> MRFVMPGDRIGSAEEYVKGEGVYEEGGELFAAVA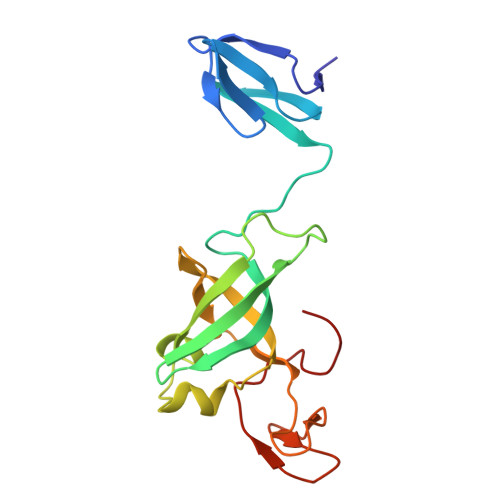GKLIIKDRVAKVESISPIPEIVKGDVVLGRVVDLRNSIALIEVSSKKGENRGPSNRGIGILHVSNVDEGYVKEISEAVGYLDILKARVIGDNLRLSTKEEEMGVLRALCSNCKTEMVREGDILKCPECGRVEKRKISTDYGKGEW> DKMDYDFKVKLSSERERVEDLFEYEGCKVGRGTYGHV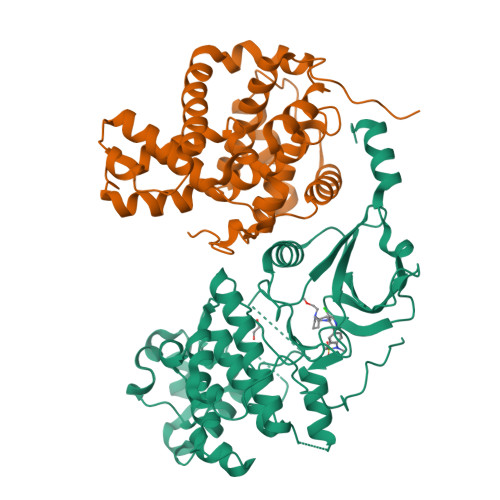YKAKRKDGKDDKDYALKQIEGTGISMSACREIALLRELKHPNVISLQKVFLSHADRKVWLLFDYAEHDLWHIIKFHRASKANKKPVQLPRGMVKSLLYQILDGIHYLHANWVLHRDLKPANILVMGEGPERGRVKIADMGFARLFNSPLKPLADLDPVVVTFWYRAPELLLGARHYTKAIDIWAIGCIFAELLTSEPIFHCRQEDIKTSNPYHHDQLDRIFNVMGFPADKDWEDIKKMPEHSTLMKDFRRNTYTNCSLIKYMEKHKVKPDSKAFHLLQKLLTMDPIKRITSEQAMQDPYFLEDPLPTSDVFAGCQIPYPKREFLTEE;> DDDDKAMAGNFWQSSHYLQWILDKQDLLKERQKDLKFLSEEEYWKLQIFFTNVIQALGEHLKLRQQVIATATVYFKRFYARYSLKSIDPVLMAPTCVFLASKVEEFGVVSNTRLIAAATSVLKTRFSYAFPKEFPYRMNHILECEFYLLELMDCCLIVYHPYRPLLQYVQDMGQEDMLLPLAWRIVNDTYRTDLCLLYPPFMIALACLHVACVVQQKDARQWFAELSVDMEKILEIIRVILKLYEQWKNFDERKEMATILSKMPKPKPPP> TRQFLIYNEDHKRCVDAVSPSAVQTAACNQDAESQKFRWVSESQIMSVAFKLCLGVPSKTDWVAITLYACDSKSEFQKWECKNDTLLGIKGEDLFFNYGNRQEKNIMLYKGSGLWSRWKIYGTTDNLCSRGYEAMYTLLGNANGATCAFPFKFENKWYADCTSAGRSDGWLWCGTTTDYDTDKLFGYCPLKFEGSESLWNKDPLTSVSYQINSKSALTWHQARKSCQQQNAELLSITEIHEQTYLTGLTSSLTSGLWIGLNSLSFNSGWQWSDRSPFRYLNWLPGSPSAEPGKSCVSLNPGKNAKWENLECVQKLGYICKKGNTTLNSFVIPSESDVPTHCPSQWWPYAGHCYKIHRDEKKIQRDALTTCRKEGGDLTSIHTIEELDFIISQLGYEPNDELWIGLNDIKIQMYFEWSDGTPVTFTKWLRGEPSHENNRQEDCVVMKGKDGYWADRGCEWPLGYICKMKSRSQGPEIVEVEKGCRKGWKKHHFYCYMIGHTLSTFAEANQTCNNENAYLTTIEDRYEQAFLTSFVGLRPEKYFWTGLSDIQTKGTFQWTIEEEVRFTHWNSDMPGRKPGCVAMRTGIAGGLWDVLKCDEKAKFVCKHWAH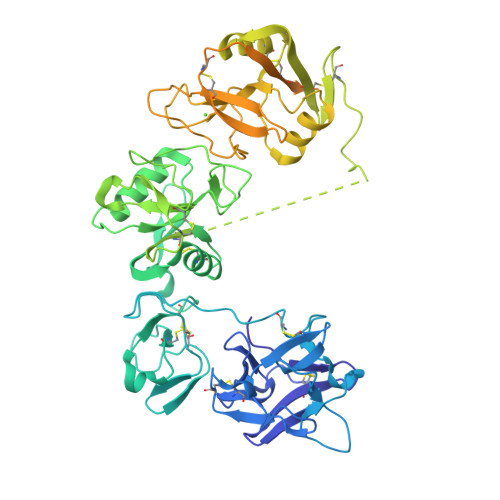HHHHH>REEEDVICDGCNGPVVGTRYKCSVCPDYDLCSVCEGKGLHRGHTKLAFPSP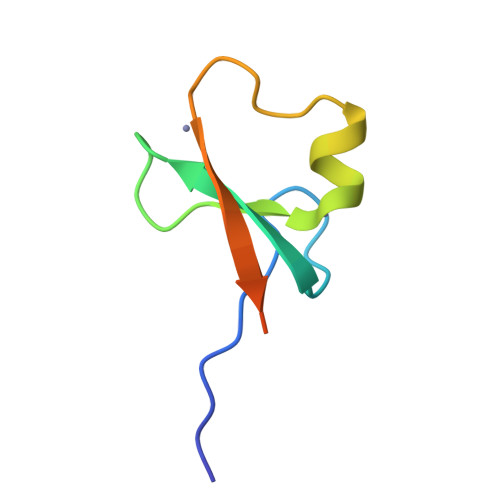FGHLSEGFS[2x]7-(5,6-DIHYDRO-8H-IMIDAZO[2,1-C][1,4]OXAZIN-2-YL)-6-FORMYL-2,7-DIHYDRO- [1,4]THIAZEPINE-3-CARBOXYLIC ACID | C13 H13 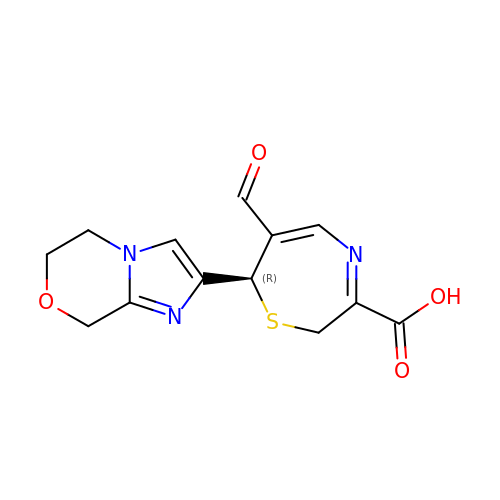N3 O4 S | CTKODGPKPNVQNS-GFCCVEGCSA-N> SMGVRKLATIRTAGEITPIAGAEAIECCHVDGWTCVIKKGEFKQGDRGVYFEIDSFIKEDNDRYPMLSKQVIDYEGQRGTRLRTARLRGQLSQGLFLPMDRFPELASNQVGDDVTEILGITKWEPPISTNLSGEILGEFPTFISKTDQERVQNLIPQIEENKGQKFEVTV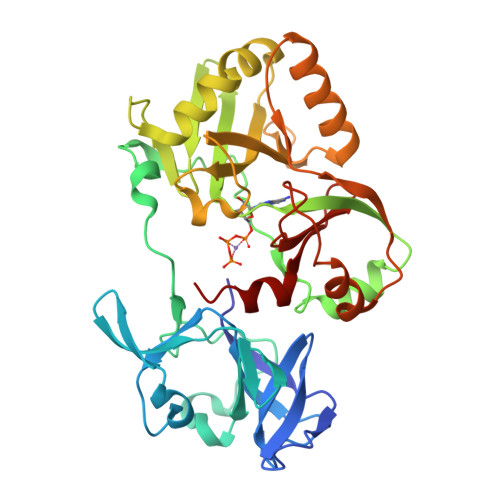KLDGSSMTVYRKDDHIGVCGRNWELRETATNAQWHAARRNKMIEGLQFLNRNLALQGAIIGESIQGNLEKLKGQDFYLFDIYDIDKAQYLTPIERQSLVKQLNDNGFTVKHVPILDDLELNHTAEQILAMADGPSLNKNVKREGLVFKRLDGKFSFKAISNAYLEKHKDR4-HYDROXYBENZALDEHYDE O-(CYCLOHEXYLCARBONYL)OXIME 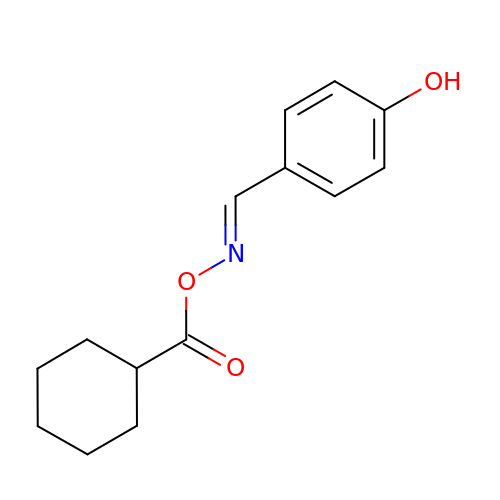| C14 H17 N O3 | YWZBYSBZDQWXGQ-XNTDXEJSSA-N> MKLYVFLVNTGTTLTFDTELTVQTVADLKHAIQS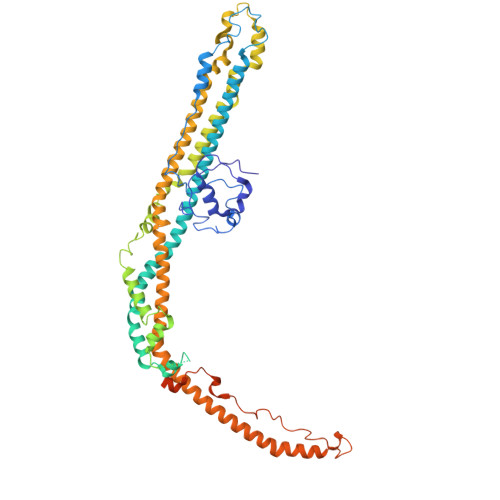KYKIAIQHQVLVVNGGECMAADRRVCTYSAGTDTNPIFLFNKEMILCDRPPAIPKTTFSTENDMEIKVEESLMMPAVFHTVASRTQLALEMYEVAKKLCSFCEGLVHDEHLQHQGWAAIMANLEDCSNSYQKLLFKFESIYSNYLQSIEDIKLKLTHLGTAVSVMAKIPLLECLTRHSYRECLGRLDSLPEHEDSEKAEMKRSTELVLSPDMPRTTNESLLTSFPKSVEHVSPDTADAESGKEIRESCQSTVHQQDETTIDTKDGDLPFFNVSLLDWINVQDRPNDVESLVRKCFDSMSRLDPRIIRPFIAECRQTIAKLDNQNMKAIKGLEDRLYALDQMIASCGRLVNEQKELAQGFLANQKRAENLKDASVLPDLCLSHANQLMIMLQNHRKLLDIKQKCTTAKQELANNLHVRLKWCCFVMLHADQDGEKLQALLRLVIELLERVKIVEALSTVPQMYCLAVVEVVRRKMFIKHYREWAGALVKDGKRLYEAEKSKRESFGKLFRKSFLRNRLFRGLDSWPPSFCTQKPRKFDCELPDISLKDLQFLQSFCPSEVQPFLRVPLLCDFEPLHQHVLALHNLVKAAQSLDEMSQTITDLLSEQK>[2x]MNKQEVILKVQECAAWWILERQSKLTKL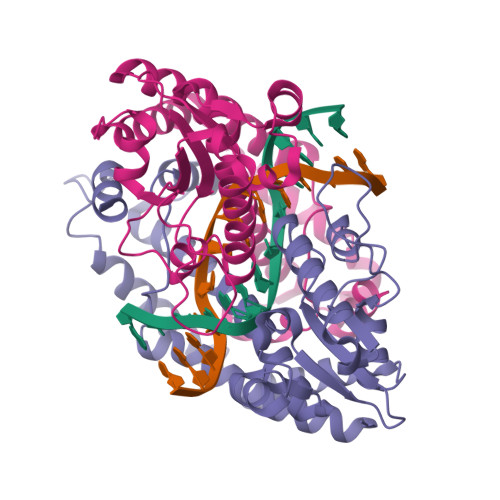MSETMSINPFMTPFIFDYHSLNDFDELVEAIIAKHLMTGHDTGFGKLIDEKILPRVFGAYKLDKSYRAANEPFIHPCFDEIDHVIQRDDGRIELLSLKAGKWTIQLTMAVQLNKAFHEIINNYPGVADNIVVGVFYGNSHGLTDKYRILRGINTGANHNVIDIRDKVHVYAGKEFWSWLNNGEAETQHWVLEGIERAVKEADIKEKNKDLIEKFKEHVAKKYNEQVLNADGTAQWHKLLEMINE2-methoxy-5-[4-[5-[(4-propan-2-ylpiperazin-1-yl)methyl]-1,3-oxazol-2-yl]-2~{H}-indazol-6-yl]pyridine-3-carboxylic acid | C25 H28 N6 O4 | 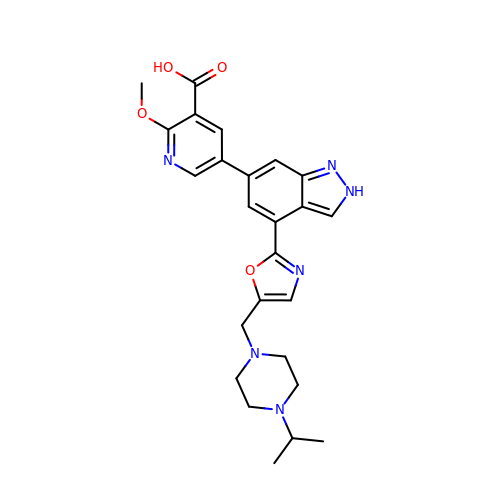CPVGTJFGSVAPTE-UHFFFAOYSA-N> PAQDNSRFVIRDRNW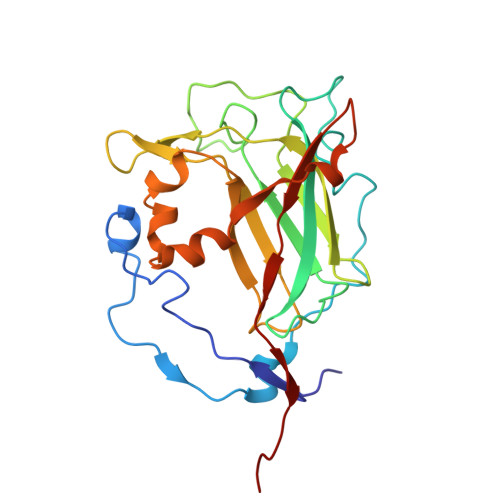HPKALTPDYKTSIARSPRQALVSIPQSISETTGPNFSHLGFGAHDHDLLLNFNNGGLPIGERIIVAGRVVDQYGKPVPNTLVEMWQANAGGRYRHKNDRYLAPLDPNFGGVGRCLTDSDGYYSFRTIKPGPHPWRNGPNDWRPAHIYFGISGPSIATKLITQLYFEGDPLIPMCPIVKSIANPEAVQQLIAKLDMNNANPMDCLAYRFDIVLRGQRKTHFENC>[5x]GDRVADVIESSIGDSVSRALTHALPAPTGQNTQVSSHRLDTGKVPALQAAEIGASSNASDESMIETRCVLNSHSTAETTLDSFFSRAGLVGEIDLPLEGTSVKRGTSVGMKPSPRPTNPNGYANWDIDITGYAQMRRKVELFTYMRFDAEFTFVACTPTGEVVPQLLQYMFVPPGAPKPDSRESLAWQTATNPSVFVKLSDPPAQVSVPFMSPASAYQWFYDGYPTFGEHKQEKDLEYGACPNNMMGTFSVRTVGTSKSKYPLVVRIYMRMKHVRAWIPRPMRNQNYLFKANPNYAGNSIKPTGASRTAITTL;>[5x]GFPTELKPGTNQFLTTDDGVSAPILPNFHPTPCIHIPGEVRNLLELCQVETILEVNNVPTNATSLMERLRFPVSAQAGKGELCAVFRADPGRSGPWQSTLLGQLCGYYTQWSGSLEVTFMFTGSFMATGKMLIAYTPPGGPLPKDRATAMLGTHVIWDFGLQSSVTLV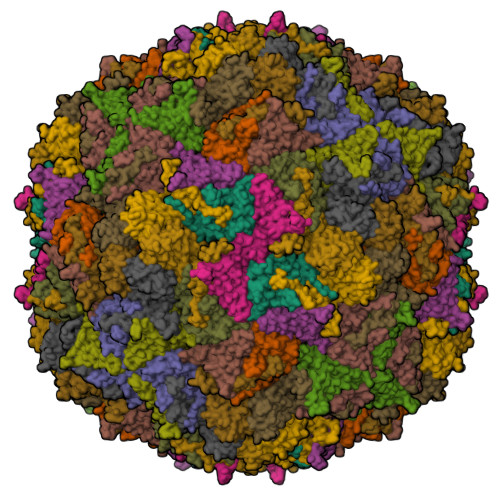IPWISNTHYRAHARDGVFDYYTTGLVSIWYQTNYVVPIGAPNTAYIIALAAAQKNFTMQLCKDASDILQTGTIQ;>MGSQVSTQRSGSHENSNSATEGSTINYTTINYYKDSYAATAGKQSLKQDPDKFANPVKDIFTEMAAPLKSPSAEACGYSDRVAQLTIGNSTITTQEAANIIVGYGEWPSYCSDSDATAVDKPTRPDVSVNRFYTLDTKLWEKSSKGWYWKFPDVLTETGVFGQNAQFHYLYRSGFCIHVQCNASKFHQGALLVAVLPEYVIGTVAGGTGTEDSHPPYKQTQPGADGFELQHPYVLDAGIPISQLTVCPHQWINLRTNNCATIIVPYINALPFDSALNHCNFGLLVVPISPLDYDQGATPVIPITITLAPMCSEFAGLRQAVTQ[5x]> GCGA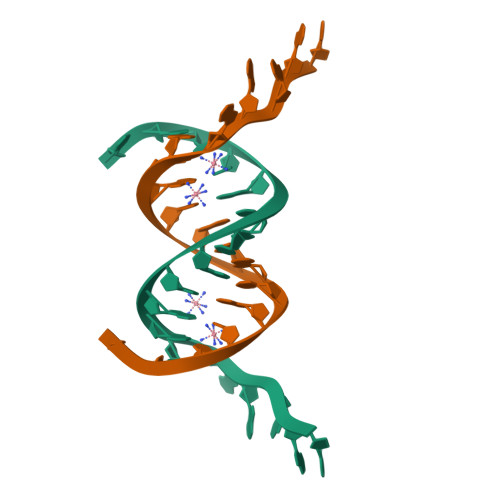AAGGGCACGTGCCCT>NNELCLRNVFTAQNTAQDFNGNESTVKSFYVTRTGKKILVAITSTKDNLKTVTCLTETGKTVLNLDPPMRFAHTVGGKQSVVYLYFIQN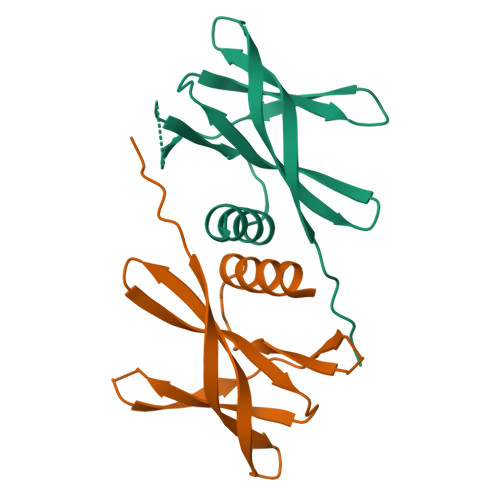ISSLNRGMVIGHISETTILQHHHHHH[4x]>[4x]THLRPYETLGAHADTMDGVTGTRFSVWAPNARRVSVVGQFNYWDGRRHPMRLRKESGIWELFIPGAHNGQLYKYEMIDANGNLRLKSDPYAFEAQMRPETASLICGLPEKVVQTEERKKANQFDAPISIYEVHLGSWRRHTDNNFWLSYRELADQLVPYAKWMGFTHLELLPINEHPFDGSWGYQPTGLYAPTRRFGTRDDFRYFIDAAHAAGLNVILDWVPGHFPTDDFALAEFDGTNLYEHSDPREGYHQDWNTLIYNYGRREVSNFLVGNALYWIERFGIDALRVDAVASMIYRDYSRKEGEWIPNEFGGRENLEAIEFLRNTNRILGEQVSGAVTMAEESTDFPGVSRPQDMGGLGFWYKWNLGWMHDTLDYMKLDPVYRQYHHDKLTFGILYNYTENFVLPLSHDEVVHGKKSILDRMPGDAWQKFANLRAYYGWMWAFPGKKLLFMGNEFAQGREWNHDASLDWHLLEGGDNWHHGV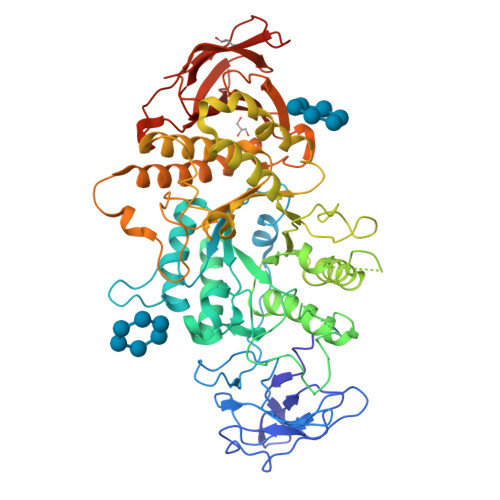QRLVRDLNLTYRHHKAMHELDFDPYGFEWLVVDDKERSVLIFVRRDKEGNEIIVASNFTPVPRHDYRFGINQPGKWREILNTDSMHYHGSNAGNGGTVHSDEIASHGRQHSLSLTLPPLATIWLVREAE> GAGCAACCUAGGAUUUUAGGCUCCCCGGCGUGUCUCGAACCAUGCCGGGCCAAACCCAUAGGGCUGGCGG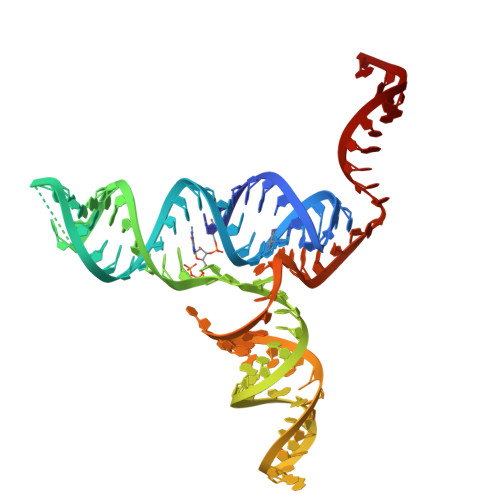UCCCUGUGCGGUCAGAAUUCAUCCGCCGGAG>[4x]PYFDNISTIAYEGPASKNPLAFKFYNPEEKVGDKTMEEHLRFSVAYWHTFTGDGSDPFGAGNMIRPWNKYSGMDLAKARVEAAFEFFEKLNIPFFCFHDVDIAPEGETLKETYKNLDIIVDMIEEYMKTSKTKLLWNTANLFTHPRFVHGAATSCNADVFAYAAAKVKKGLEIAKRLGAENYVFWGGREGYETLLNTDMKLELDNLARFLHMAVDYAKEIGFDGQ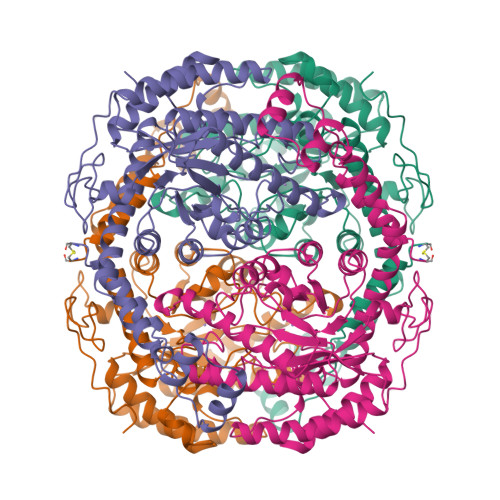FLIEPKPKEPTKHQYDFDVATALAFLQTYGLKDYFKFNIEANHATLAGHTFEHELRVARIHGMLGSVDANQGDMLLGWDTDEFPTDLYSTTLAMYEILKNGGLGRGGLNFDAKVRRGSFEPEDLFYAHIAGMDSFAVGLKVAHRLIEDRVFDEFIEERYKSYTEGIGREIVEGTADFHKLEAHALQLGEIQNQSGRQERLKTLLNQYLLEVCAAR> PDLTDQPIPDADYTWYTDGSSFLQEGQRRAGAAVTTETEVIWARA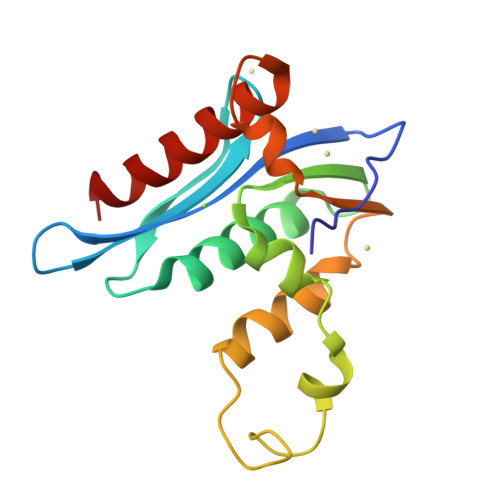LPAGTSAQRAELIALTQALKMAEGKKLNVYTDSRYAFATAHVHGEIYRRRGLLTSEGREIKNKNEILALLKALFLPKRLSIIHCPGHQKGNSAEARGNRMADQAAREAAMKA[(2R,3S,4R,5R)-5-(6-azanyl-8-oxo-7H-purin-9-yl)-3,4-dihydroxy-oxolan-2-yl]methyl phosphono hydrogen phosphate | C10 H15 N5 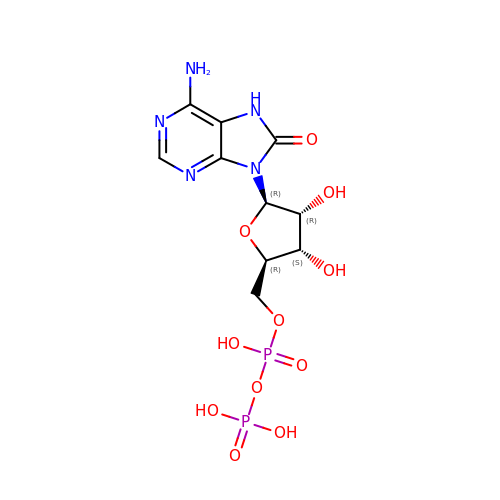O11 P2 | RKHXUJRVBUXHAN-UUOKFMHZSA-N> MLDAFSRVVVNSDSKAAYVSGS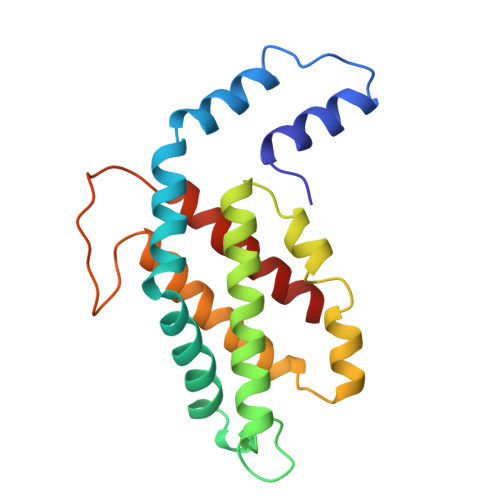DLQALKTFINDGNKRLDAVNYIVSNSSCIVSDAISGMICENPGLITPGGNCYTNRRMAACLRDGEIILRYVSYALLAGDASVLEDRCLNGLKETYIALGVPTNSTVRAVSIMKAAAVCFISNTASQRKVEVIEGDCSALASEVASYCDRVVAAVS> RGSHMLEMIIKPRVRGFICVTAHPTGCEANVKKQIDYVTTEGPIANGPKRVLVIGASTGYGLAARITAAFGCGADTLGVFFERPGEEGKPGTSGWYNSAAFHKFAAQKGLYAKSINGDAFSDEIKQLTIDAIKQDLGQVDQ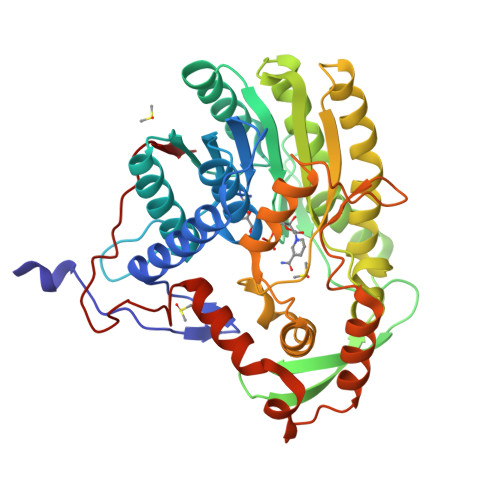VIYSLASPRRTHPKTGEVFNSALKPIGNAVNLRGLDTDKEVIKESVLQPATQSEIDSTVAVMGGEDWQMWIDALLDAGVLAEGAQTTAFTYLGEKITHDIYWNGSIGAAKKDLDQKVLAIRESLAAHGGGDARVSVLKAVVVQASSAIPMMPLYLSLLFKVMKEKGTHEGCIEQVYSLYKDSLCGDSPHMDQEGRLRADYKELDPEVQNQVQQLWDQVTNDNIYQLTDFVGYKSEFLNLFGFGIDGVDYDADVNPDVKIPNLIQG>MSIIAINENGFLDKIKGRNPLFTCVISSIETTLSIPISGVHRDVIKYTPSADVELVFYGKSLTLKTPPIDATGSPTPATITRACVELKNIKNLHIDAGAFVKPKIPFIEIDEKPTGRIEEGKAMNNSKELYMKGYLLGKNLDAELLIVGESVPGGTTTALGVLLGLGYDAEGKVSSGSINNPHELKIKVVREGLKKAGINEKSSVFDVLNAVGDKMMPVVAGLAISFAERNKPVILAGGTQMSAVLAVIKEINKKVLDKNLIAIGTTEFVLN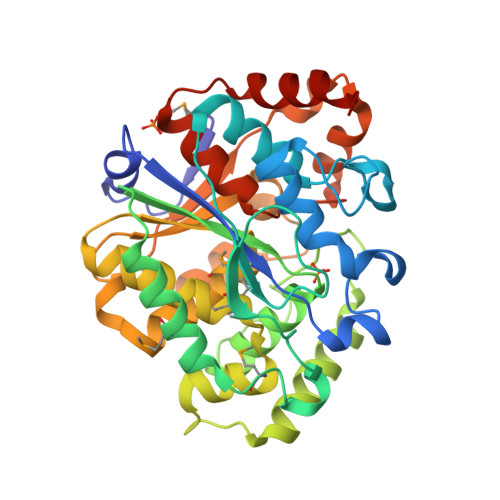DKKGDLKGIVEQIGNVPVLASKFYFEKAKIEGLKNYCKGSVKEGVGAGGIAVYSIVNDLEPTKIREFIENKFYEWYKE[3x]> NVHSNYTFIIAGGGISGLTLADRLTEDPRVTVLVIEAGPLDRGEDGILVPGAFSPWLYFWPGLVSTPQAGLNNRTVDVITAQVVGGGSTINAMVYLRGDKDDYDSWG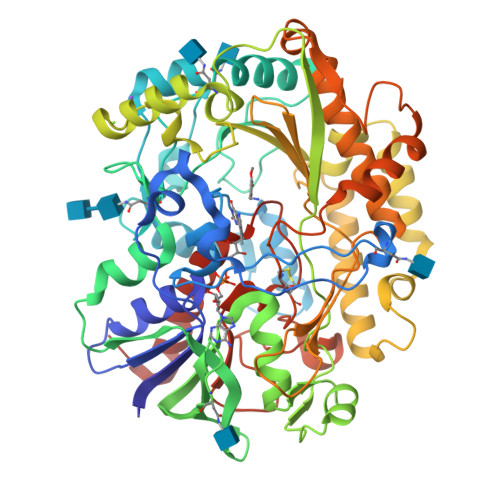ALGNPGWSWNSMLPYFIKSETFTPPSPELAAAGNITWDGSIRGRSGPVNYSYPNYFFPGSENWWNAANEVGLPPVKDPMAGSKQGVFWIPSAIDARTMTRSHARRNHYDRVSSRPNYHILPSHLVSKILFRGKQAIGVSYIPTSGGNTTTNVYASKEITLAAGGLGTPKILQLSGIGPRKLLNELGIPVISDLPGVGQNLQDQPTLTIPYTFTNNVFPNTDSLTTNATYNAEQRALYDSSKQGAYTIVNSLSTNIGVMSLQRAAPKSYRQIIAAARARSASLSLPPGTDPAVIRGYQAQRNAILKQFENPNVGVGTVHWGTGSSALVYHLKPLSRGTVNIRSTNPLDAPEIDYRTGTDPIDAQVYTSLFRKNREIFNAPSMRVLGPSEAAPFGANLTTDEEIYAVMRELINPSNAHQCCTAAMMPKDMGGVVSSEQKVYGVQGLRVADISFWPFQLSGSPMATAYAGAERLADVIKKEHRLAGAPKSL>MEIPGSLCKKVKLSNNAQNWGMQRATNVTYQAHHVSRNKRGQVVGTRGGFRGCTVWLTGLSGAGKTTVSMALEEYLVCHGIPCYTLDGDNIRQGLNKNLGFSPEDREENVRRIAEVAKLFADAGLVCITSFISPYTQDRNNARQIHEGASLPFFEVFVDAPLHVCEQRDVKGLYKKARAGEIKGFTGIDSEYEKPEAPELVLKTDSCDVNDCVQQVVELLQERDIVPVDASYEVKELYVPENKLHLAKTDAETLPALKINKVDMQWVQVLAEGWATPLNGFMREREYLQCLHFDCLLDGGVINLSVPIVLTATHEDKERLDGCTAFALMYEGRRVAILRNPEFFEHRKEERCARQWGTTCKNHPYIKMVMEQGDWLIGGDLQVLDRVYWNDGLDQYRLTPTELKQKFKDMNADAVSAFQLRNPVHNGHALLMQDTHKQLLERGYRRPVLLLHPLGGWTKDDDVPLMWRMKQHAAVLEEGVLNPETTVVAIFPSPMMYAGPTEVQWHCRARMVAGANFYIVGRDPAGMPHPETGKDLYEPSHGAKVLTMAPGLITLEIVPF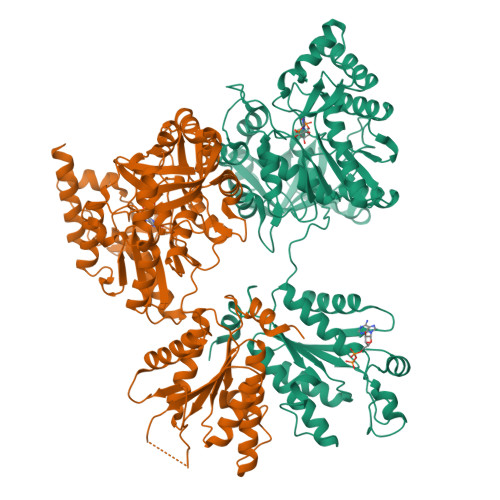RVAAYNKKKKRMDYYDSEHHEDFEFISGTRMRKLAREGQKPPEGFMAPKAWTVLTEYYKSLEKAHHHHHH[2x]Peptidyl-prolyl isomerases (PPIases) catalyze cis/trans isomerization of peptidyl-prolyl bonds, which is often rate-limiting for protein folding. SlyD is a two-domain enzyme containing both a PPIase FK506-binding protein (FKBP) domain and an insert-in-flap (IF) chaperone domain. In order to improve our understanding of the mechanism of SlyD and of FKBPs in general, we set out to analyze the kinetics, energetics, and structural basis for substrate binding and inhibition of SlyD from Thermus thermophilus (TtSlyD) using 15-residue-long unmodified peptides, which we reasoned would be better mimics of natural unfolded protein substrates than the traditionally used 4-nitroanilide tetrapeptides. In total, we obtained five structures of TtSlyDFL and three of TtSlyDΔIF at a maximum resolution of up to 1.4 Å.

Finally, we also analyzed binding of the S2, S3, and mutated variants of the S2 peptide to a chimeric TtSlyD construct, in which the IF domain is replaced by the flap loop from human FKBP12 (henceforth abbreviated TtSlyDΔIF). Next, we tested binding of an S2 mutant peptide where the sole tryptophan residue was replaced by alanine (S2-W23A). This peptide retained the ability to bind to both domains of TtSlyDFL, albeit with moderately reduced affinities. The binding mode is the same for both TtSlyDFL molecules in the TtSlyDFL:S2 structure, whereas the S2-W23A peptide binds in two different ways to the four molecules in the TtSlyDFL:S2-W23A structure: one similar to the S2 peptide (molecules A and C), and one in a different but partially overlapping fashion (molecules B and D). This latter binding mode was also observed in the TtSlyDΔIF:S2-W23A structure. However, our results speak against such a scenario, because both type VIa1 and distorted VIb β-turns are observed in our TtSlyDFL:S2, TtSlyDFL:S2-W23A, and TtSlyDΔIF:S2-W23A structures, which strongly suggests that FKBPs can catalyze cis/trans isomerization of prolines present in (at least) both these two types of β-turns. As discussed further below, this variability is intimately connected with interactions between the side chain of Y63 and the peptides bound to the FKBP domain. The FKBP12 flap loop inserted into TtSlyDΔIF in place of the IF domain adopts essentially the same conformation as in full-length FKBP12 in the case of TtSlyDΔIF:FK506, while it is partially disordered in TtSlyDΔIF:S2-W23A and TtSlyDΔIF:S3.

> MKVGQDKVVTIRYTLQVEGEVLDQGELSYLHGHRNLIPGLEEALEGREEGEAFQAHVPAEKAYGATGHPGIIPPHATLDFQVEVVKVREATPEELLHGHAHPSGHHHHHH;> TRYANPKMKPFIFGAX> MEVEKEFITDEAKELLSKDKLIQQAYNEVKTSICSPIWPATSKTFTIN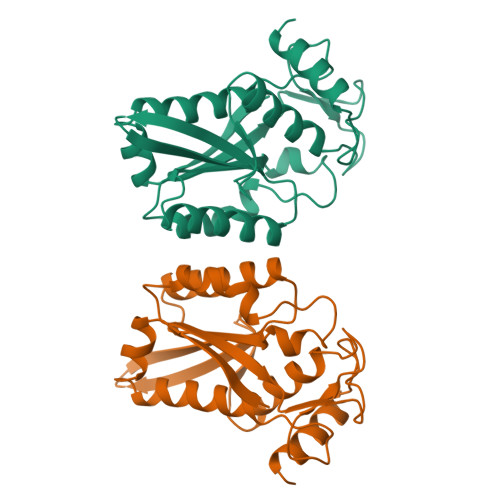NTEKNCNGVVPIKELCYTLLEDTYNWYREKPLDILKLEKKKGGPIDVYKEFIENSELKRVGMEFETGNISSAHRSMNKLLLGLKHGEIDLAIILMPIKQLAYYLTDRVTNFEELEPYFELTEGQPFIFIGFNAEAYNSNVPLIPKGSDGMSKRSIKKWKDKVENK>[2x]VDSVYRTRSLGVAAEGLPDQYADGEAARVWQLYIGDTRSRTAEYKAWLLGLLRQHGCHRVLDVACGTGVDSIMLVEEGFSVMSVDASDKMLK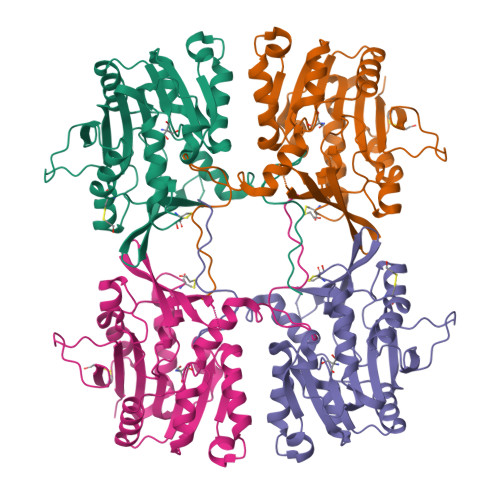YALKERWNRRKEPSFDNWVIEEANWLTLDKDVLSGDGFDAVICLGNSFAHLPDCKGDQSEHRLALKNIASMVRPGGLLVIDHRNYDYILSTGCAPPGKNIYYKSDLTKDITTSVLTVNNKAHMVTLDYTVQVPGTGRDGSPGFSKFRLSYYPHCLASFTELVRAAFGGRCQHSVLGDFKPYKPGQAYVPCYFIHVLKKTD>MAHHHHHHVDDDDKMRTRSTISTPNGITWYYEQEGTGPDVVLVPDGLGECQMFDSSVSQIAAQGFRVTTFDMPGMSRSAKAPPETYTEVTAQKLASYVISVLDALDIKHATVWGCASGASTVVALLLGYPDRIRNAMCHELPTKLLDHLSNTAVLEDEEISKILANVMLNDVSGGSEAWQAMGDEVHARLHKNYPVWARGYPRTIPPSAPVKDLEALRGKPLDWTVGAATPTESFFDNIVTATKAG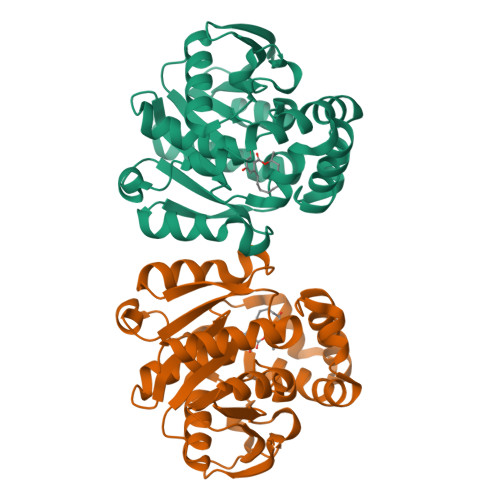VNIGLLPGMHFPYVSHPDVFAKYVVETTQKHL[3x]>SMRYRQITIPRGKDGFGFTICCDSPVRVQAVDSGGPAERAGLQQLDTVLQLNERPVEHWKCVELAH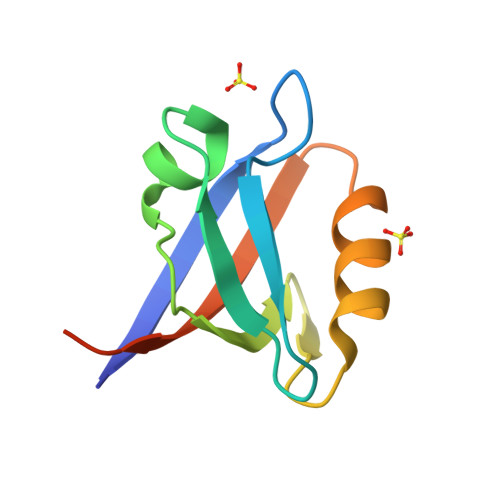EIRSCPSEIILLVWRMVPQVKPGPD[2x]> PSSPTSEIGRHLAQLGDSYSV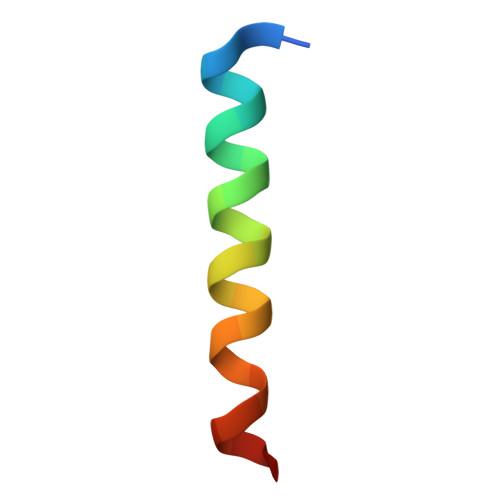RFQNE> AKCVSYGVSQIKAPALHSQGYTGSNVKVAVIDSGIDSSHPDLNVAGGASFVPSETNPFQDNNSHGTHVAGTVLAVAPSASLYAVKVLGADGSGQYSWII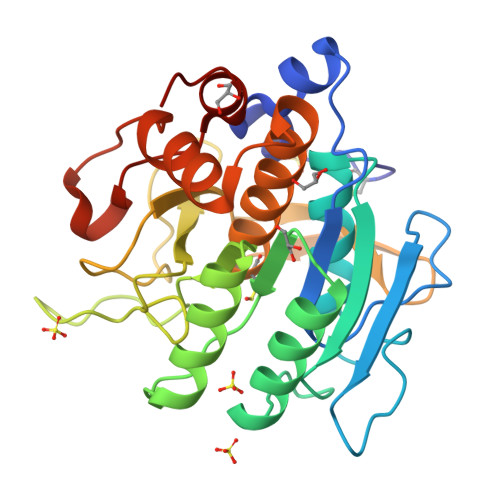NGIEWAIANNMDVINMSLGGPSGSAALKAAVDKAVASGVVVVAAAGNSGTSGSSSTVSYPAKYPSVIAVGAVDSSNQRAPFSSVGPELDVMAPGVSICSTLPGNKYGAHSGTCPASAHVAGAAALILSKHPNWTNTQVRSSLENTATKLGDSFYYGKGLINVEAAAQHHHHHH> DDRDLLLAPKWISFLSLSSFLKQKLLSLLRQIRELRLTTTVYPPQDKLMWWSHCCDPEDIKVVILGQDPYHKGQATGLAFSVDPQCQVPPSLRSIFRELEASVPNFSTPSHGCLDSWARQGVLLLNTVLTVEKGRAGSHEGLGWDWFTSFIISSISSKLEHCVFLLWGRKAIDRTPLINAQKHLVLTAQHPSPLASLGGR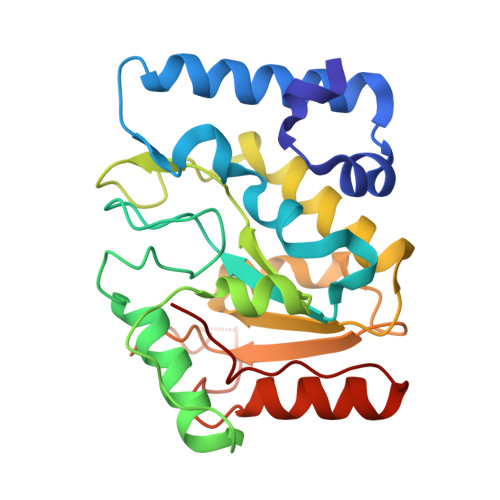HSRWPRFQGCNHFNLANDYLTRHRRETVDWGLLEQ> GHMEPGDAGIYHHEGHRIRLTKDGRCIITCKTVEVYADESMTVDTPRTTFTGDVEIQKGLGVKGKSQFDSNITAPDAIINGKSTDKHIHRG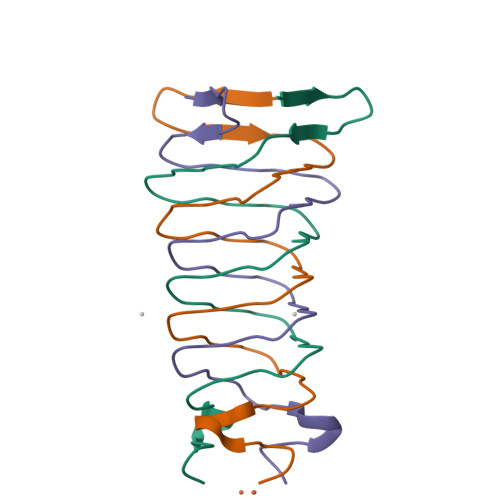DSGGTTGPMQ>MSLANQTTKTLGLVMPSSASKAFQNPFFPEVIRGISSFAHVEGYALYMSTGETEEEIFNGVVKMVQGRQIGGIILLYSRENDRIIQYLHEQNFPFVLIGKPYDRKDEITYVDNDNYTAAREVAEYLISLGHKQIAFIGGGSDLLVTRDRLAGMSDALKLADIVLPKEYILHFDFSRESGQQAVEELMGLQQPPTAIMATDDLIGLGVLSALSKKGFVVPKDVSIVSFNNALLSEIASPPLSTVDVNIYQLGYEAAKALVDKVENAESTAKCIIIPHKLLKRQTCEGHHHHHH[2x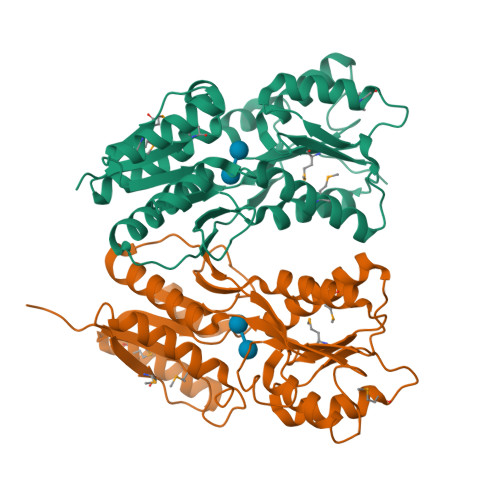]>[2x]MKVAVLPGDGIGPEVTEAALKVLRALDEAEGLGLAYEVFPFGGAAIDAFGEPFPEPTRKGVEEAEAVLLGSVGGPKWDGLPRKIRPETGLLSLRKSQDLFANLRPAKVFPGLERLSPLKEEIARGVDVLIVRELTGGIYFGEPRGMSEAEAWNTERYSKPEVERVARVAFELARKRRKHVVSVDKANVLEVGEFWRKTVEEVGRGYPDVALEHQYVDAMAMHLVRSPARFDV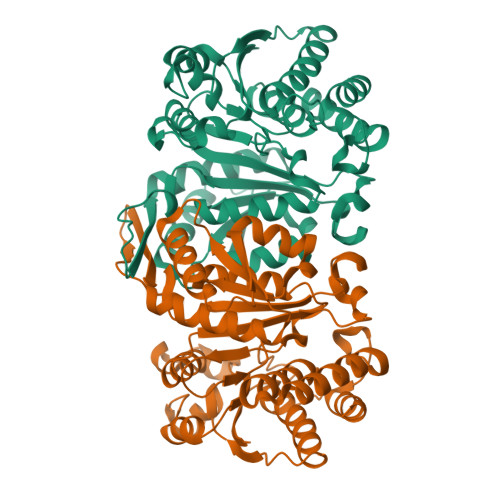VVTGNIFGDILSDLASVLPGSLGLLPSASLGRGTPVFEPVHGSAPDIAGKGIANPTAAILSAAMMLEHAFGLVELARKVEDAVAKALLETPPPDLGGSAGTEAFTATVGMGI>RKTYTLTDYLKNTYRLKLYSLRWISDHEYLYKQENNILVFNAEYGNSSVFLENSTFDEFGHSINDYSISPDGQFILLEYNYVKQWRHSYTASYDIYDLNKRQLITEERIPNNTQWVTWSPVGHKLAYVWNNDIYVKIEPNLPSYRITWTGKEDIIYNGITDWVYEEEVFSAYSALWWSPNGTFLAYAQFNDTEVPLIEYSFYSDESLQYPKTVRVPYPKAGAVNPTVKFFVVNTDSLSSVTNATSIQITAPASMLIGDHYLCDVTWATQERISLQWLRRIQNYSVMDICDYDESSGRWNCLVARQHIEMSTTGWVGRFRPSEPHFTLDGNSFYKIISNEEGYRHICYFQIDKKDCTFITKGTWEVIGIEALTSDYLYYISNEYKGMPGGRNLYKIQLSDYTKVTCLSCELNPERCQYYSVSFSKEAKYYQLRCSGPGLPLYTLHSSVNDKGLRVLEDNSALDKMLQNVQMPSKKLDFIILNETKFWYQMILPPHFDKSKKYPLLLDVYAGPCSQKADTVFRLNWATYLASTENIIVASFDGRGSGYQGDKIMHAINRRLGTFEVEDQIEAARQFSKMGFVDNKRIAIWGWSYGGYVTSMVLGSGSGVFKCGIAVAPVSRWEYYDSVYTERYMGLPTPEDNLDHYRNSTVMSRAENFKQVEYLLIHGTADDNVHFQQSAQISKALVDVGVDFQAMWYTDEDHGIASSTAHQHIYTHMSHFIKQCFSLP[2x];> TECDFSPMFKGVAPQVYNFKRLVFSNCNYNLTKLLSLFAVDEFSCNGISPDAIARGCYSTLTVDYFAYPLSMKSYIRPGSAGNIPLYNYKQSFAHPTCRVLASVPPNVTITKPEAYGYISKCSRLTGDYQHIETPLYINPGEYSICRDFAPLGFSEDGQVFK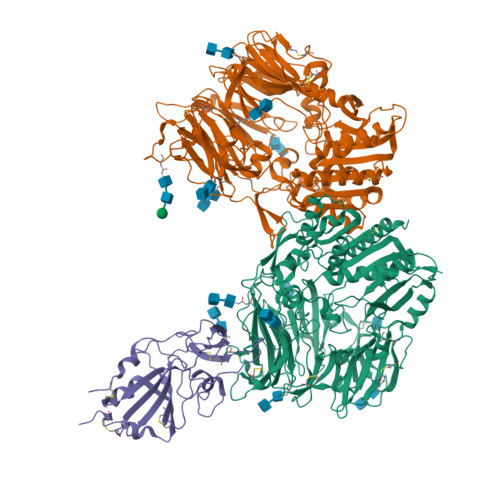RTLTQFEGGGLLIGVGTRVPMTANLEMGFVISVQYGAGTDSVCPMLD>CPRFLKVKNWETDVVLTDTLHLKSTLETGCTEHICMGSIMLPSQHTRKPEDVATKDQLFPLAKEFLDQYYSSIKRFGSKAHMDRLEEVNKEIESTSTYQLKDTELIYGAKHAWRNASRCVGRIQWSKLQVFDARDCTTAHGMFNYICNHVKYATNKGNLRSAITIFPQRTDGKHDFRVWNSQLIRYAGYKQPDGSTLGDPANVQFTEICIQQGWKAPRGRFDVLPLLLQANGNDPELFQIPPELVLEVPIRHPKFDWFKDLGLKWYGLPAVSNMLLEIGGLEFSACPFSGWYMGTEIGVRDYCDNSRYNILEEVAKKMDLDMRKTSSLWKDQALVEINIAVLYSFQSDKVTIVDHHSATESFIKHMENEYRCRGGCPADWVWIVPPMSGSITPVFHQEM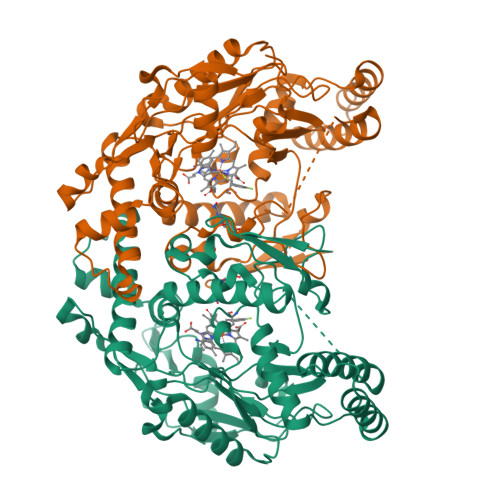LNYRLTPSFEYQPDPWNTHVWKG[2x]>[6x]MEKIKVAIADDNKELVKTLESYLADHPQIEVITTAPNGKVILSLMENDLPDVLLLDIIMPHLDGLAVLEMMQANENLSKVQVIMLT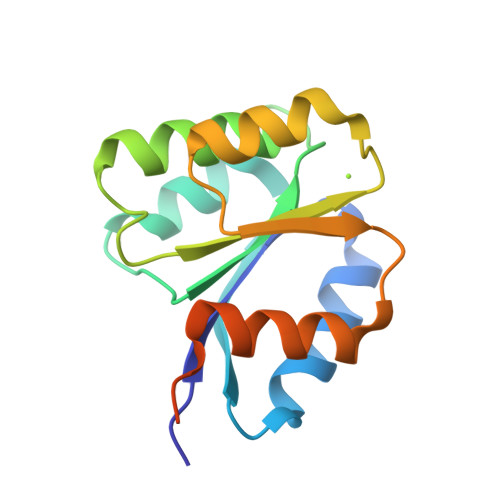AFGQEDVMKQAVDLGASYFMLKPFEFDRLVNQILQVAGHKQEADQRSSILQSQPQPKT;> GSHMMEKIKVAIADDNKELVKTLESYLADHPQIEVITTAPNGKVILSLMENDLPDVLLLDIIMPHLDGLAVLEMMQANENLSKVQVIMLTAFGQEDVMKQAVDLGASYFMLKPFEFDRLDNQILQVAGHKQEADQRSSILQSQPQPKT> DDT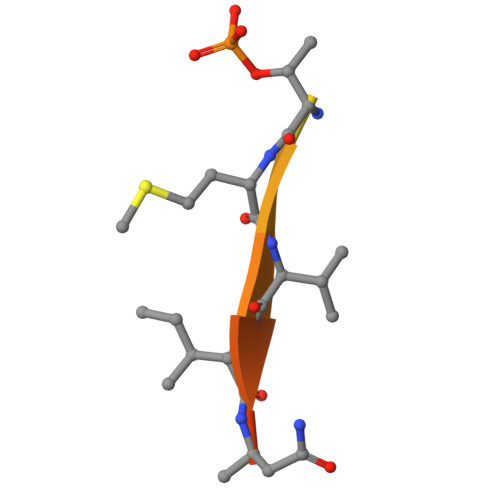LPSQLGTMVINAED>AVTGQVDVKLNISTGCTVGGSQTEGNMNKFGTLNFGKTSGTWNNVLTAEVASAATGGNISVTCDGTDPVDFTVAIDGGERTDRTLKNTASADVVAYNVYRDA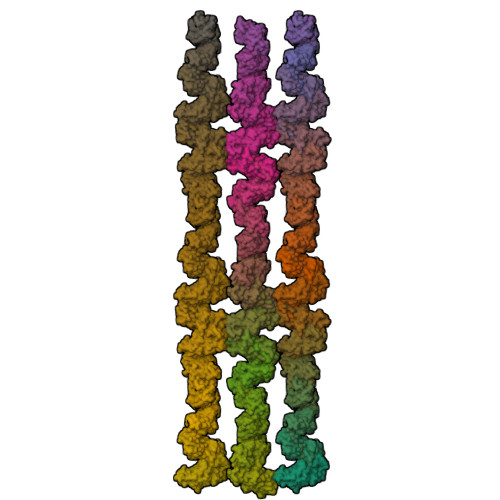ARTNLYVVNQPQQFTTVSGQATAVPIFGAIAPNTGTPKAQGDYKDTLLVTVNF[57x]> MSSRFFQKYFIRCGNCQTIQRYAKGYKPIPNPILFDSDAHCRSYHRERRDCTGLTGTLVTCRCDKCARVHSHWTVMDFQEFLDAKLVMTPEERTALL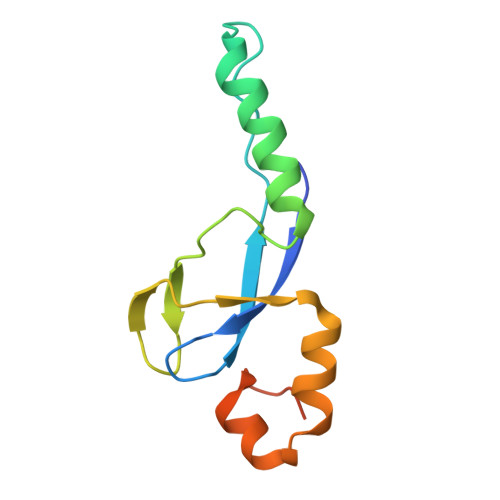WPGAGSRAEPSSGTSN2-(hydroxymethyl)butane-1,4-diol 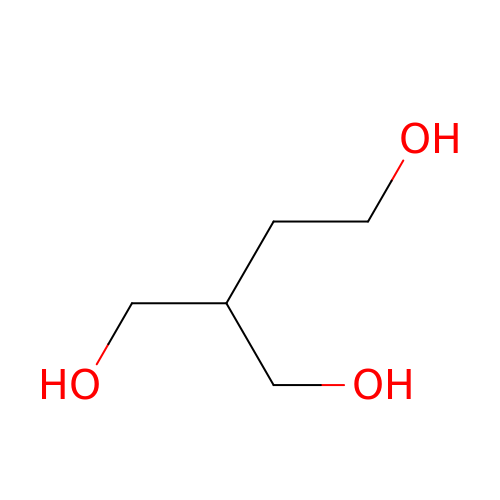| C5 H12 O3 | SYNPRNNJJLRHTI-UHFFFAOYSA-N>[2x]TKNPKLFISSTWMSHMTMPTENTDGEESLTSSKQQQQQSGDKHMEPLGTDDDFWGPSGPVSTEVVDRERNLYRVRLPMAGSYHCPSTGLHFVVTRAVTIEIGFCAWSQFLHETPLQHSHMVAGPLFDIKAEHGAVTAVCLPHFVSLQEGKVDSSLFHVAHFQDHGMVLETPARVEPHFAVLENPSF;>SPMGVLLRMIPAVGHFIPITSITLIYYRLYLEDITFHLYLVPNDCTIRKAIDEEELKFQFVRINKPPPVDALYVGSRYIVSSSKEVEILPKELELCYRSPRESQLFSEIYVGNIGSGINLQLTDKKYMNLIWEALLKPGDLRPALPRMASAPKD[2x]

Nucleotide-binding domain, leucine-rich repeat receptors (NLRs) mediate innate immunity by forming inflammasomes. Activation of the NLR protein NLRP1 requires autocleavage within its function-to-find domain (FIIND). In resting cells, the dipeptidyl peptidases DPP8 and DPP9 interact with the FIIND of NLRP1 and suppress spontaneous NLRP1 activation; however, the mechanisms through which this occurs remain unknown. Here we present structural and biochemical evidence that full-length rat NLRP1 (rNLRP1) and rat DPP9 (rDPP9) form a 2:1 complex that contains an autoinhibited rNLRP1 molecule and an active UPA–CARD fragment of rNLRP1.

A crystal structure of the rNLRP1 FIIND of rNLRP1 shows that the purified protein is autocleaved at the predicted position between F968 and S969. This is further confirmed by SDS–PAGE analysis of the crystals. The structure of rNLRP1 FIIND resembles that of the autoinhibited netrin receptor UNC5b. Inter-domain interaction between ZU5 and UPA largely involves the first β-strand (β13) of UPA, which forms two anti-β sheets with ZU5; this explains how the ZU5 domain can block the release of the active UPA–CARD fragment. The catalytically essential FS motif20 is conserved in NLRP1 homologues and in CARD8. H942 of rNLRP1, which is highly conserved in NLRP1 proteins and in CARD8, is located adjacent to S969 from the FS motif. Collectively, these data suggest that H942 of rNLRP1 is a catalytic residue.> EQARPADDALAALGAQLFVDPALSRNATQSCATCHDPARAFTDPREGKAGLAVSVGDDGQSHGDRNTPTLGYAALVPAFHRDANGKYKGGQFWDGRADDLKQQAGQPMLNPVQMAMPDRAAVAARLRDDPAYRTGFEALFGKGVLDDPERAFD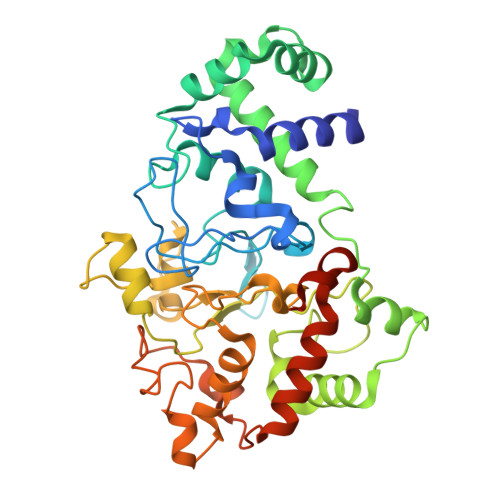AAAEALAAYQATGEFSPFDSKYDRVMRGEEKFTPLEEFGYTVFITWNCRLCHMQRKQGVAERETFTNFEYHNIGLPVNETAREASGLGADHVDHGLLARPGIEDPAQSGRFKVPSLRNVAVTGPYMHNGVFTDLRTAILFYNKYTSRRPEAKINPETGAPWGEPEVARNLSLAELQSGLMLDDGRVDALVAFLETLTDRRYEPLLEESRAAQKDHHHHHH> MTTQLRYENNDDDERVEYNLFTNRSTMMANFEEWIKMATDNKINSRNSWNFALIDYFYDLDVLKDGENNINFQKASATLDGCIKIYSSRVDSVTTETGKLLSGLAQRKTNGASNGDDSNGGNGEGLGGDSDEANIEIDPLTGMPISNDPDVNNTRRRVYNRVLETTLVEFETIKMKELDQELIIDPLFKKALVDFDEGGAKSLLLNTLNIDNTARVIFDASIKDTQNVGQGKLQRKEEELIERDSLVDDENEPSQSLISTRNDSTVNDSVISAPSMEDEILSLGMDFIKFDQIAVCEISGSIEQ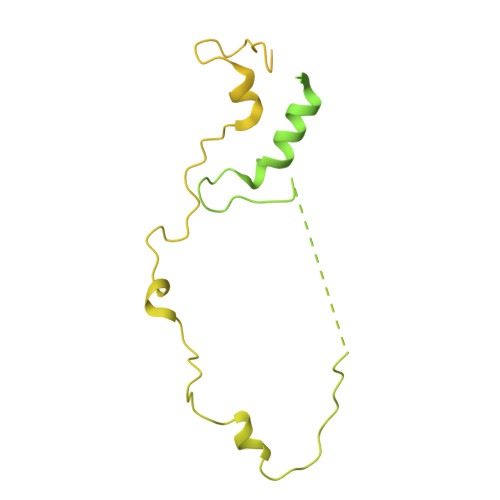LRNVVEDINQAKDFIENVNNRFDNFLTEEELQAAVPDNAEDDSDGFDMGMQQELCYPDENHDNTSHDEQDDDNVNSTTGSIFEKDLMAYFDENLNRNWRGREHWKVRNFKKANLVNKESDLLEETRTTIGDTTDKNTTDDKSMDTKKKHKQKKVLEIDFFKTDDSFEDKVFASKGRTKIDMPIKNRKNDTHYLLPDDFHFSTDRITRLFIKPAQKMSLFSHRKHTRGDVSSGLFEKSTVSANHSNNDIPTIADEHFWADNYERKEQEEKEKEQSKEVGDVVGGALDNPFEDDMDGVDFNQAFEGTDDNEEASVKLDLQDDEDHKFPIRENKVTYSRVSKKVDVRRLKKNVWRSINNLIQEHDSRKNREQSSNDSETHTEDESTKELKFSDIIQGISKMYSDDTLKDISTSFCFICLLHLANEHGLQITHTENYNDLIVNYEDLATTQAASLVGGGHHRPHHGGHHHHHHGGRIFYPYDVPDYAGYPYDVPDYAGSYPYDVPNYAAGH>[8x]GPMAK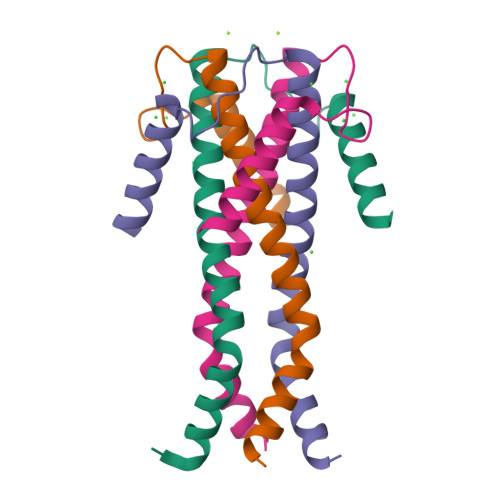VKKHLTFSGPTESPYGIAYIEKEMKAKNCSKMNETIELIFAEHDEMKARLSEQDALVEKIFQRFKKTLDVIRVRAGHTDKNAQINLELWNAFLMANPLPVTVLTDQHTSESVSMAKEKVSNDIATFKQRKDEQKAKQEMQKGEK>[2x]LQVDIVPSQGEISVGESKFFLCQVAGDAKDKDISWFSPNGEKLTPNQQRISVVWNDD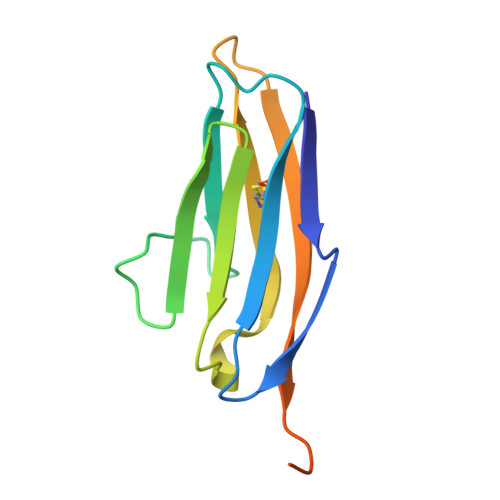SSSTLTIYNANIDDAGIYKCVVTGEDGSESEATVNVKIFQAAADYKDDDDKAADYKDDDDK>PENITFDTLNTQNDHEETYGESPEVPKASIAPAGRQNVPVLQQNQENEDNHALGGSEDAKDEREIQSSAIKTLYNYYSEGPSTPIMPHLVNRLRGLDALAKVDATLSKVDMNAAYIFALRPTFPYSYGYKQRFSNRRLTTSALCYARTGLSSFLTVDKTYTSNSPLKGGSRGWPIFNVGVSPHVAEPHMRTLSPIGLEVFNLATSQFSKTLLTASSKVFTQSLYTADILSIFGEVFLPHVMQPVSNYTPILVRALLALIHILGSGSGNCSLSSSIFESSIPQFLTISHSTNMSNRTRYCLHTWSAYKDMFRNGIPPQSTFPPTLAPEGSSARILIPAALVTSPMFPWLLVLVSSGPQFFLYSKDASINTVDIGSRGRITSPIPDVAHLDLHRLWNLFRFDGYRYIDVVIVGVDRDYVWPYQNGVYVHGGKGPKGTDNYENADVHDGIGTIFSSFNNNVNVQTSDLLLGLSTLWNHITTTYATEEEVTMAIKIAAAFALVYPVQPIVYSGCSRALYNHTSYFQPSSENCYTTDTAEVKSTWDTVELSVQVNNAMVLGMTLPFGQPTVSSAQWFNNIDKAEISMFKVGNLPLQNLDYLSLDMMEFYAPTTGQLYDIRSDSLISSAHRTVNLGIGYTALADFFAYLASVPAQSFYHNRMVTSPISKQAYSVYERFIERFIDDFVGWGRCDLFNLDTLLGAKRIAGVASSPIPWHCSLQRCPLPIIMHYTGLHFGQEHIRVRDVAGVEGLQQIVLRNDQGSIVLDALGTAAPSRLAVKLDWSRLSAWYSDTTCAIPISDRVMEIVNYAAIWDPTQERRATGFVYTYFSPNFLSSFNVSEPIFNKTINLTPPYDDTSQTVIQNLSMPQMLSFDPYYESTFYVVSADNEWVPTSGPAWKVPYLENVVKRSGRRLLAELRIASNNGSGDRTFLDDV[2x]

The double-stranded (ds)RNA virus Giardia lamblia virus (GLV or Giardiavirus) exclusively infects G. duodenalis. ORF1 expresses a capsid protein (CP) that assembles an icosahedral capsid. The GLV capsid comprises 60 copies of CP dimers named subunits A and B (CP-A and CP-B) in the triangulation number (T) = 1 icosahedral asymmetric unit. The overall structure of the GLV CP shows a typical α-helix-rich α+β fold commonly adopted in the Totiviridae and other icosahedral dsRNA viruses.

The first high-resolution capsid structure of two GLV subtypes was determined using cryogenic electron microscopy (cryo-EM) single-particle analysis at a resolution of 2.1 Å and 2.6 Å for GLV-HP and GLV-CAT, respectively. As confirmed in our observations, the GLV-HP particles tend to aggregate with each other both within giardia parasite cells and in purified samples, whereas the GLV-CAT particles do not exhibit this behavior. Additionally, chronic infection of GLV-HP hampers parasite growth more markedly than GLV-CAT, indicating that GLV-HP might have features of a pre-lytic virus. However, only the CP-B to CP-A direction is identified in the GLV-HP capsid. This C-terminal interlocking includes three possible hydrogen bonds: Arg671–Asp922, Arg675–Asp928, and Lys774–Asp927 in CP-B to CP-A in GLV-HP. However, apparent structural differences are observed between GLV-HP and GLV-CAT CP-A/CP-B dimers. The major structural difference of CP-A is the aforementioned absence of C-terminal extension in GLV-HP, while that of CP-B is a variable loop that consists of Pro316–Ser330 residues, localizing between the interface of CP-B and that of CP-A. Notably, Phe320 in GLV-HP forms intrasubunit interactions with Val184, Leu590, and Asn592 in the CP-B; however, in GLV-CAT, the corresponding Leu320 in CP-B interacts with Asn112 and Gln282 residues in the adjacent CP-A. The GLV-HP particles interact with each other, which causes particle aggregation and affects the preferable intracellular localization. Nano differential scanning fluorimetry (nanoDSF) thermographs differences in Ti (inflection temperature) values between GLV-HP and GLV-CAT particles, which may reflect their capsid stability in multiple dissociation or unfolding steps. It is also another possibility that a lack of intersubunit interactions, which are mediated by the variable loops within the GLV-HP capsid, might instead allow intersubunit interactions between two virions. The comparative analysis of the two GLV prototypes reveals significant conformational differences in the C-terminal extension and the variable loop, which are critical for CP–CP interactions. It is hypothesized that the loose assembly of the CPs in GLV-HP could expose hydrophobic CP–CP interfaces to facilitate particle–particle interactions.> MTCTTGAGVTSGFIDLATYDNLDRALYGGKDATTYFIKEHYPVGWFTKLPTMATRVSGNPAFGQEFSVGVPRSGDYVLNAWLTLKTPEIKLLETNRLG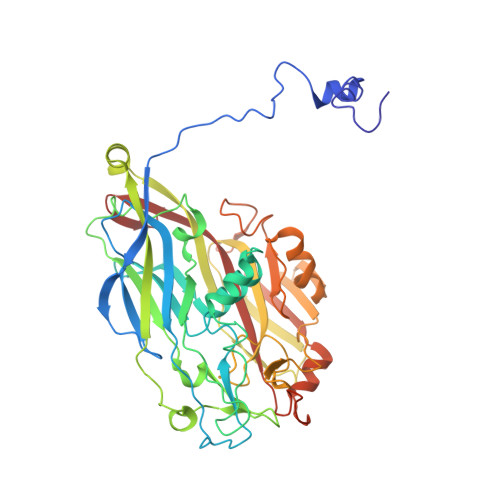ANGTVRWTKNLMHNAVEHASLTFNDICAQQFNTAYLDAWTQFNMCEGKRIGYDNMIGNTSDMTNPTPAQGQDGARTLPSKNLVLPLPFFFSRDCGLALPTVVLPYNEIRINIKLRSLQELLVFQNKDTGNVIPISATDIAGGLADTVEAYVYMTVGLVSNVERCAMAGTVRDMVVEQMQAAPTHIVNPQNTNNVHVDMRFSHAVKALFFMVQNVTYKSVGSNYTCVTPVNGPGNTVMEPAMSVDPIKSASLTYENTTRLANMGVEYYSLVQPWYFSASIPVYTGYHMYSYALNVGSVHPSGSTNYGRLTNASITVTMSPESVVAAAGGGNNNSGYNEPQRFALVVIAVNHNVIRIMNGSMGFPIL> SNQKKVGVTSKSEVFEFLTHLVKQEPDLLTRIYCFQPITMND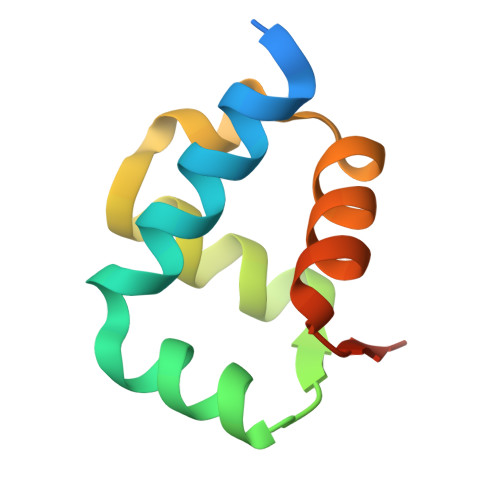LINKLRNKDSFVDLIDDGTIREWTDKLGICIRSNNLKD> GSQKERLLDELTLEGVARYMQSERCRRVICLVGAGISTSAGIPDFRSPSTGLYDNLEKYHLPYPEAIFEISYFKKHPEPFFALAKELYPGQFKPTICHYFMRLLKDKGLLLRCYTQNIDTLERIAGLEQEDLVEAHGTFYTSHCVSASCRHEYPLSWMKEKIFSE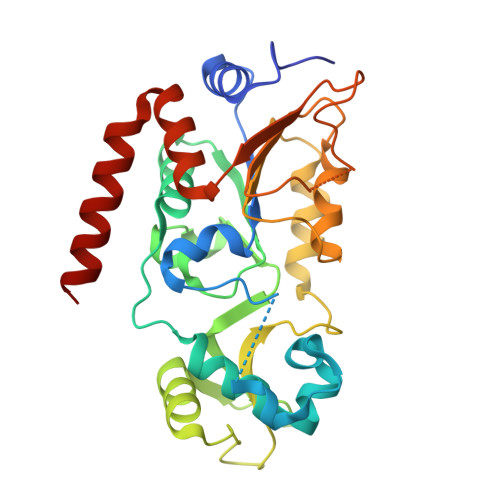VTPKCEDCQSLVKPDIVFFGESLPARFFSCMQSDFLKVDLLLVMGTSLQVQPFASLISKAPLSTPRLLINKEKAGGGGMDFDSKKAYRDVAWLGECDQGCLALAELLGWKKELEDLVRREHASIDAQS> GAMGSGLAKYLPGATNLLSKSGEVSLGSLVGKTVFLYFSASWCPPCRGFTPVLAEFYEKHHVAKNFEVVLISWDENESDFHDYYGKMPWLALPFDQRSTVSEL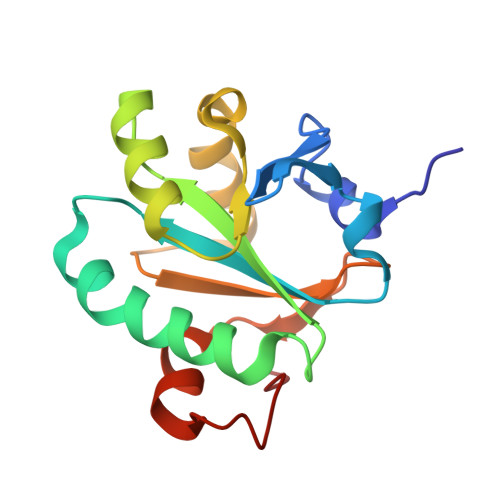GKTFGVESIPTLITINADTGAIIGTQARTRVIEDPDGANFPWPN> MAQILPIRFQEHLQLQNLGINPANIGFSTLTMESDKFICIREKVGEQAQVVIIDMNDPSNPIRRPISADSAIMNPASKVIALKAGKTLQIFNIEMKSKMKAHTMTDDVTFWKWISLNTVALVTDNAVYHWSMEGESQPVKMFDRHSSLAGCQIINYRTDAKQKWLLLTGISAQQNRVVGAMQLYSVDRKVSQPIEGHAASFAQFKMEGNAEESTLFCFAVRGQAGGKLHIIEVGTPPTGNQPFPKKAVDVFFPPEAQNDFPVAMQISEKHDVVFLITKYGYIHLYDLETGTCIYMNRISGETIFVTAPHEATAGIIGVNRKGQ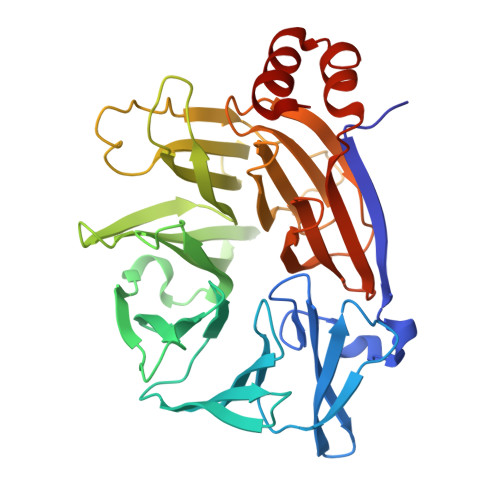VLSVCVEEENIIPYITNVLQNPDLALRMAVRNNLAG>GEGSVLEQIDQGSILKLPSNLLFENATSDAINQDMMLYIERIAKIIQKLPKRVHINVRGFTDDTPLVKTRFKSHYELAANRAYRVMKVLIQYGVNPNQLSFSSYGSTNPIAPNDSLENRMKNNRVEIFFSTDANDLSKIHSILDNEFNPHKQQE[2x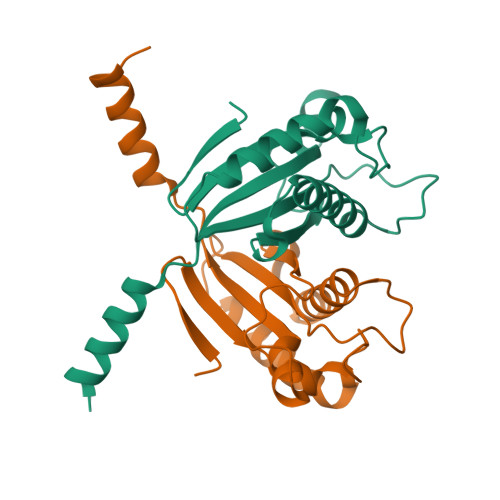]>GPHMLEVPPQPQYSYHDINVYSLAGLAPHITLNPTIPL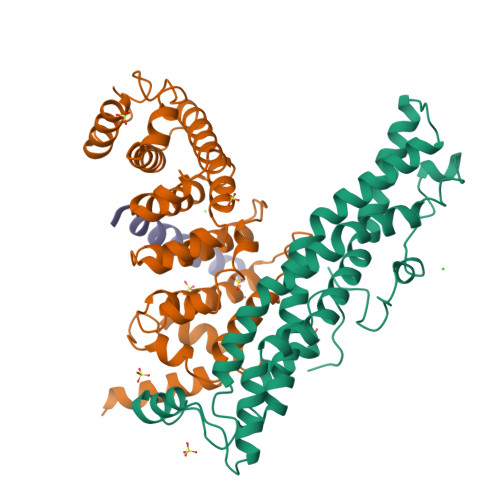FQAHPQLKQCVRQAIERAVQELVHPVVDRSIKIAMTTCEQIVRKDFALDSEESRMRIAAHHMMRNLTAGMAMITCREPLLMSISTNLKNSFASALRTASPQQREMMDQAAAQLAQDNCELACCFIQKTAVEKAGPEMDKRLATEFELRKHARQEGRRYCDPVVLTYQAERMPEQIRLKVGGVDPKQLAVYEEFARNVPGFLPTNDL[2x];>[2x]GPHMLEREKIYQWINELSSPETRENALLELSKKRESVPDLAPMLWHSFGTIAALLQEIVNIYPSINPPTLTAHQSNRVCNALALLQCVASHPETRSAFLAAHIPLFLYPFLHTVSKTRPFEYLRLTSLGVIGALVKTDEQEVINFLLTTEIIPLCLRIMESGSELSKTVATFILQKILLDDTGLAYICQTYERFSHVAMILGKMVLQLSKEPSARLLKHVVRCYLRLSDNPRAREALRQCLPDQLKDTTFAQVLKDDTTTKRWLAQLVKNLQE;>DDQQLDHNFKQMEEHLALMVEGNE[2x]> AGFCEVCKKLVGYLDRNLEKNSTKQEILAA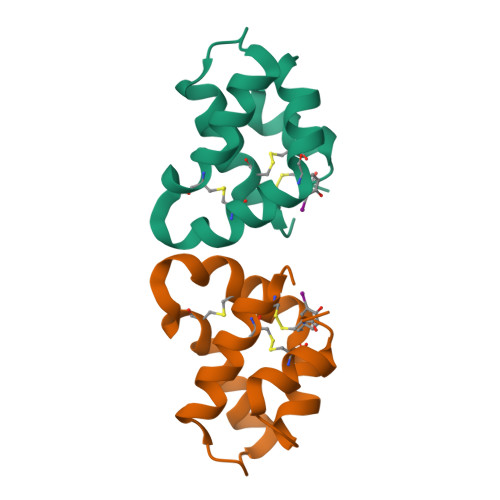LEKGCSFLPDPYQKQCDQFVAEYEPVLIEILVEVMDPSFVCLKIGACPSHHHHHH>XXXXXXXXXXXXXXXXXXXXCDTDSETLYDLMTQHWHLKTPNLVISVTGGAKNFALKPRMRKIFSRLIYIAQSKGAWIFTGGTHYGLMKYIGEVVRDNTISRSSEENVVAIGIAXXXXXLKRDPLYCLDNNHTHLLLVDNGTHGHPTIEAKVRTQLEKYISERVIPESNYGGKIPIVCFAQGGGKETLKSINVAIKSKIPCVVVEGSGRIADVIASLVEAEGTLASSCVKESLLRFLPRTISRLSEEETESWIKWIKEVLESPHLLTVIKIEEAGDEIVSNAISFALYKAFSTNEHDRDNWNGQLKLLLEWNQLDLASDEIFTNDRNWESADLQDVMFTALVKDRPKFVRLFLENGLNLRKFLTTEVLRELYTNNFSSLVFKNLQIAKNSYNDALLTFVWKMVEDFRRGAKRDDKNSKDEMEIELSEECPITRHPLQALFIWSVLQNKKELSKVIWEQTRGCTLAALGASKLLKSMAKVKNDINAAGESEELANEYETRAVELFTECYSNDEDLAEQLLTYSCEAWGGSNCLELAVEARDQQFIAQPGVQNFLSKQ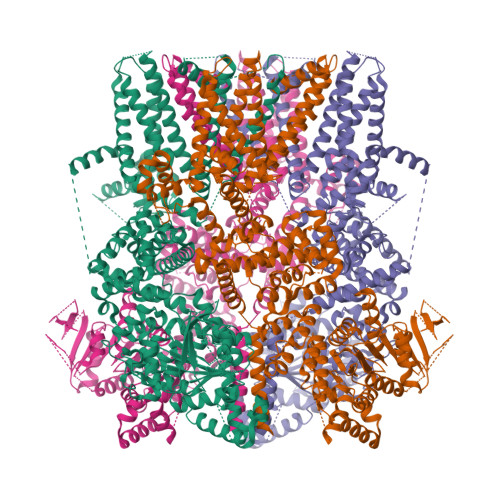WYGEISRDTKNWKIILCLFFFPLIGCGFISFRKKPVEKTKKLFLYYVSFFTSPFVVFSWNVIFYIAFLLLFAYVLLMDFQKEPTALEIILYVLVFILLCDEVRQWYMNGSKYFSDLWNVMDTLAIFYFIAGIVFRLHSDESSWYSGRVIFCLDYIVFTLRLIHIFTVSRNLGPKIIMLQRMMIDVFFFLFLFAVWMVAFGVARQGILRKNEHRWEWIFRSVIYEPYLAMFGQYPDDIDGTTYNFDHCTFSGNESKPLCVELDANNQPRFPEWITIPLVCIYMLSTNILLVNLLVAMFGYTVGSVQENNDQVWKFQRFFLVQEYCSRLTXXXXXXXXXXXXXXXXXXRNEDNEILAWEAVMKENYLVKINTXXXXXXXXXXXXXXXXXXXXXXXX[4x]(7S,10aR)-1-methyl-4-{4-[(5R)-1,1,5-trihydroxy-4,4-dimethyl-1,6,11-trioxo-2-oxa-7,10-diaza-1lambda~5~-phosphadodecan-12-yl]phenyl}-3,5,6,7,8,9,10,10a-octahydrocycloocta[d]pyridazin-7-yl 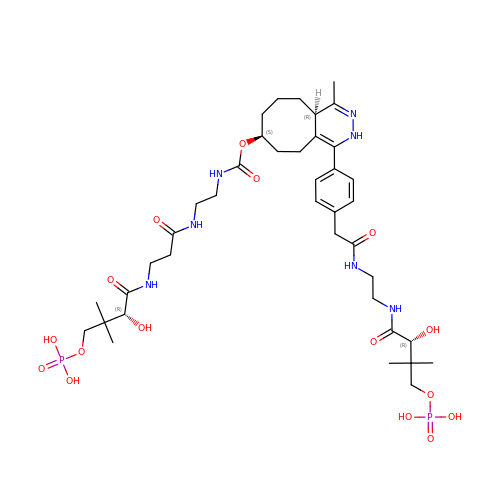[2-({N-[(2R)-2-hydroxy-3,3-dimethyl-4-(phosphonooxy)butanoyl]-beta-alanyl}amino)ethyl]carbamate | C39 H63 N7 O16 P2 | YOLLUOFJIOLVFE-XKJABPBFSA-N>MRVLALSAVFLVASIIGMPAVAKEWQENKSWNAHFTEHKSQGVVVLWNENKQQGFTNNLKRANQAFLPASTFKIPNSLIALDLGVVKDEHQVFKWDGQTRDIAAWNRDHDLITAMKYSVVPVYQEFARQIGEARMSKMLHAFDYGN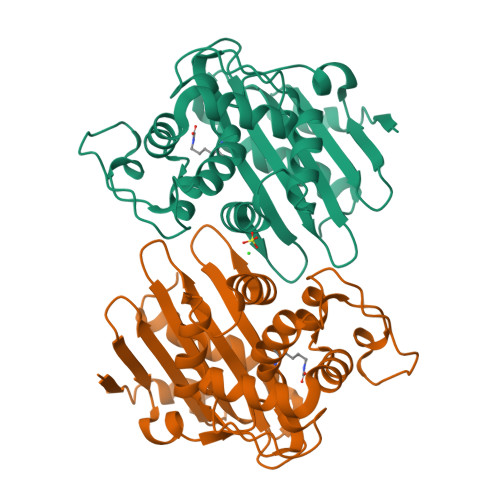EDISGNVDSFWLDGGIRISATQQIAFLRKLYHNKLHVSERSQRIVKQAMLTEANGDYIIRAKTGYSTRIEPKIGWWVGWVELDDNVWFFAMNMDMPTSDGLGLRQAITKEVLKQEKIIP[2x]>[8x]LYWDDLKRKLSEKLDSTDFTSTIKLLNENSYVPREAGSQKDENLALYVENEFRE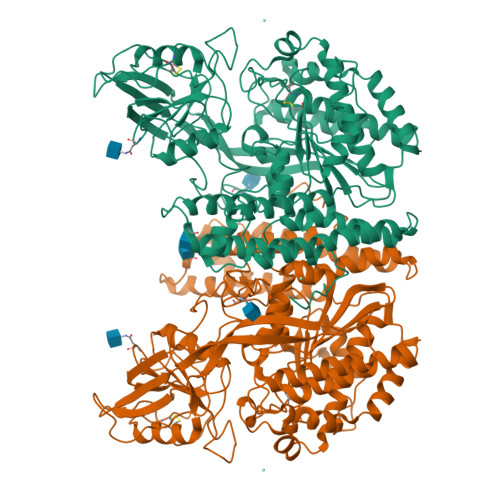FKLSKVWRDQHFVKIQVKDSAQNSVIIVDKNGRLVYLVENPGGYVAYSKAATVTGKLVHANFGTKKDFEDLYTPVNGSIVIVRAGKITFAEKVANAESLNAIGVLIYMDQTKFPIVNAELSFFGHAHLGTGDPYTPGFPSFNHTQFPPSRSSGLPNIPVQTISRAAAEKLFGNMEGDCPSDWKTDSTCRMVTSESKNVKLTVSNVLKEIKILNIFGVIKGFVEPDHYVVVGAQRDAWGPGAAKSGVGTALLLKLAQMFSDMVLKDGFQPSRSIIFASWSAGDFGSVGATEWLEGYLSSLHLKAFTYINLDKAVLGTSNFKVSASPLLYTLIEKTMQNVKHPVTGQFLYQDSNWASKVEKLTLDNAAFPFLAYSGIPAVSFCFCEDTDYPYLGTTMDTYKELIERIPELNKVARAAAEVAGQFVIKLTHDVELNLDYEEYNSQLLSFVRDLNQYRADIKEMGLSLQWLYSARGDFFRATSRLTTDFGNAEKTDRFVMKKLNDRVMRVEYHFLSPYVSPKESPFRHVFWGSGSHTLPALLENLKLRKQNNGAFNETLFRNQLALATWTIQGAANALSGDVWDIDNEF Type IV pili (T4P)1 are long, surface-exposed filaments which extend from the surfaces of bacterial cells. T4P are composed of both major and minor pilin components, although major pilins comprise the majority of the pilin subunits within each fibre. We identified a cluster of type IV pilin-like genes within the T. thermophilus HB8 genome, using the program PilFind. Three of the remaining six, TTHA1218, TTHA1219 and TTHA1222, yielded crystals of truncated forms which enabled us to solve their structures (designated here as Tt121836-123, Tt121933-236 and Tt122238-123).

Although the structure of Tt121836-123 identifies it as recognizably part of the pilin family, it exhibits a different fold topology from Tt122238-123. The first β-strand is formed from the loop between the α-helix and what would be β1 in Tt122238-123. Formation of this strand may be assisted by a disulphide bond which links the loop to β2 in Tt121836-123 (which is β1 in Tt122238-123). This location is similar to the conserved disulphide observed in TTHA1221 and Tt122238-123, hinting that this may be a common structural feature of Thermus pilins. The structure also contains a second disulphide bond, which links β2 and β3 in the equivalent location to the D loop. Both Tt121836-123 and Tt122238-123 form 4-stranded β-sheets, but the location of the strands is displaced between the two: a short α-helix and β1 in Tt121836-123 are formed in place of the loop between the α-helix and β1 in Tt122238-123; β2 in Tt121836-123 aligns with β1 in Tt122238-123, and there is no equivalent of β4 from Tt122238-123 in Tt121836-123. Our results show that TTHA1218 and TTHA1219 are closer in structure to T2SS pseudopilins than to other type IV pilins for which structures are currently available. In P. aeruginosa, the type IV core minor pilins, FimU, PilV, PilW and PilX, are clustered in an operon; determination of the crystal structure of FimU revealed close similarity to the T2SS pseudopilin GspH, despite the low sequence homology between the two proteins. This work complements our observations reported here, in that we have identified two type IV pilins from Thermus which are most closely related at a structural level to two other T2SS pseudopilins, GspI and GspJ. To test whether Tt121836-123 and Tt121933-236 could plausibly form a heterodimer, we modelled both structures on to their GspI/J counterparts in the GspIJK structure. Inspection of the structure suggested that its formation is plausible but would require two structural changes to alleviate minor steric clashes.

> MAGQQGRELQTVVREMENFMERLRQDPQGIPALCNGALALGGKQGTCTAIPCNVAQDGGLACPTAGDVRAFQVVLRVEEKRLETVVYRPLEHHHHHH> XGA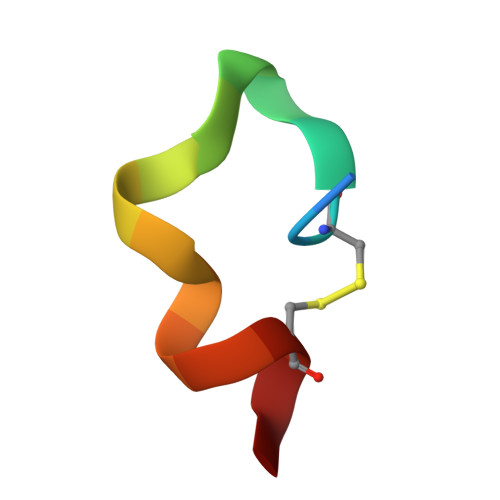CGLGQEEWFWLCAA>ALQPRRVS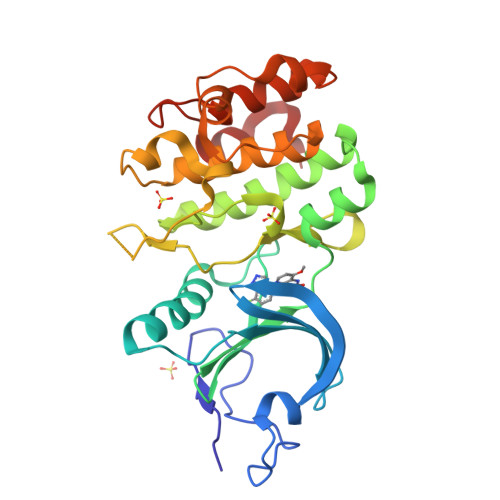FRGEASETLQSPGYDPSRPESFFQQSFQRLSRLGHGSYGEVFKVRSKEDGRLYAVKRSMSPFRGPKDRARKLAEVGSHEKVGQHPCCVRLEQAWEEGGILYLQTELCGPSLQQHCEAWGASLPEAQVWGYLRDTLLALAHLHSQGLVHLDVKPANIFLGPRGRCKLGDFGLLVELGTAGAGEVQEGDPRYMAPELLQGSYGTAADVFSLGLTILEVACNMELPHGGEGWQQLRQGYLPPEFTAGLSSELRSVLVMMLEPDPKLRATAEALLALPVLRQ[2x]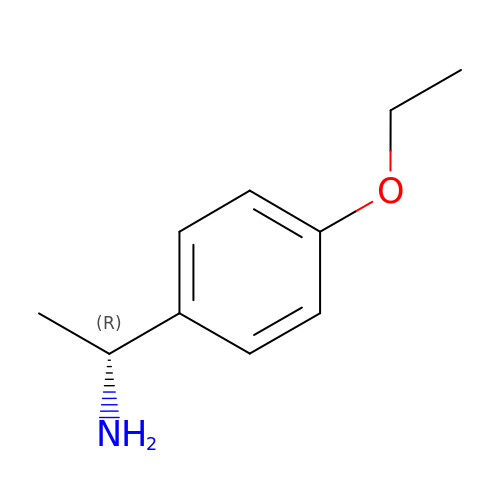(1~{R})-1-(4-ethoxyphenyl)ethanamine | C10 H15 N O | LQISONQSSGPXMA-MRVPVSSYSA-N N-methyl-N-[(2S,3R,4R,5R)-2,3,4,5,6-pentakis(oxidanyl)hexyl]nonanamide | C16 H33 N O6 | 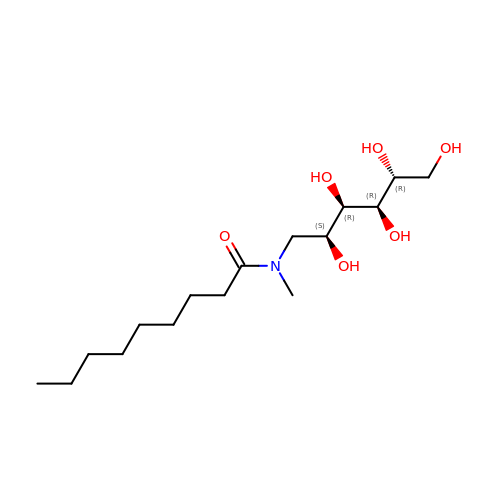GCRLIVCNZWDCDE-SJXGUFTOSA-N>[3x]MKVFVVLAAIVAIANGLTSGSGVTTRYWDCCKPSCSWGGKASVTKPV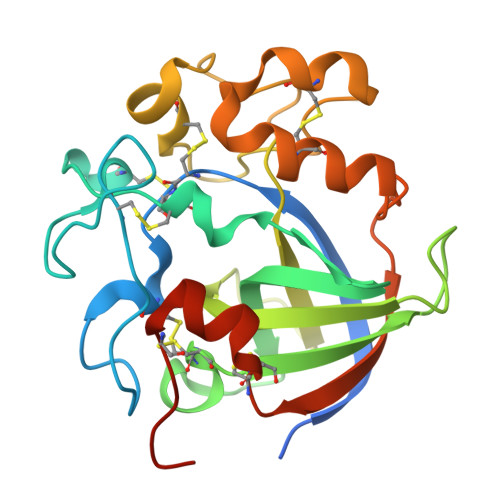RTCKANGNTTIDSNTQSGCNGGSSYVCNDQQPFTQGNVGYGFAAASISGQPESQTCCACYEMTFTNTAISGQKMIVQVTNTGSDLNGNHFDLMIPGGGVGIFNGCQSQWGAPSNGWGQRYGGISSQSECNQLPTSLRAGCNWRFGWFKNADNPSMKFTQVRCPTILTQKSQCVRTPGPHHHHHH> TTPIVHLKGDANTLKCLRYRFKKHCTLYTAVSSTWHWTGH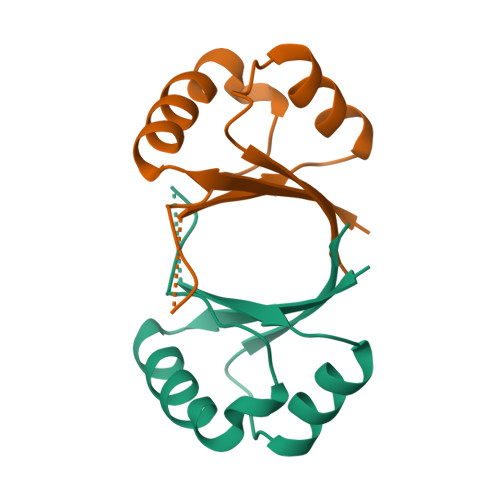NVKHKSAIVTLTYDSEWQRDQFLSQVKIPKTITVSTGFMSI L-URIDINE-5'-MONOPHOSPHATE 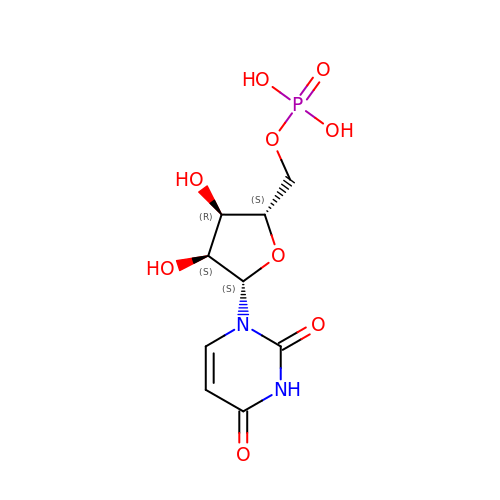| C9 H13 N2 O9 P | DJJCXFVJDGTHFX-PSQAKQOGSA-N Plant nucleotide-binding leucine-rich repeat receptors (NLRs) are intracellular receptors that play a key role in the plant innate immune system by sensing the presence of pathogen effectors delivered inside plant cells during pathogenesis through direct or indirect recognition. Sr35 was first identified in a landrace of the Triticum urartu relative Triticum monococcum (einkorn) and confers immunity to Pgt Ug99 in bread wheat when transferred as a transgene. Direct effector binding to the leucine-rich repeats of Sr35 results in the formation of a pentameric Sr35–AvrSr35 complex, which we term the Sr35 resistosome. Electrophysiological measurements show that the Sr35 resistosome exhibits non-selective cation channel activity.

To circumvent cell death activation for protein purification, we introduced substitutions in the N-terminal residues L15E/L19E (Sr35L15E/L19E), which are predicted to be essential for Sr35 membrane association by analogy with the ZAR1 resistosome. The final 3D reconstruction of the Sr35–AvrSr35 complex contains five receptor protomers, each bound to one effector molecule. As in the ZAR1 resistosome, five Sr35 NOD modules define the base of the circular protomer arrangement, and a helical barrel formed by the fivecoiled-coil domains is buried at the centre. Unlike ZAR1, the leucine-rich repeat (LRR) domains at the outer region do not pack against each other in the Sr35 resistosome, which might explain why this region is more flexible. The modelled ATP is nested in a groove formed by HD1 and NBD. Instead, the γ-phosphate group of the ATP forms a bidentate hydrogen bond with Sr35 NBDR157 and NBDR311. Of note, the coiled-coil domain of Sr35 contributes considerably to the interprotomer interactions: the C-terminal half of α4-helix from one protomer packs against the C-terminal sides of α2- and α4-helices of the neighbouring coiled-coil protomer. In the cryo-EM structure of the Sr35 resistosome, the EDIVD motif (Glu-Asp-Ile-Val-Asp) and the adjacent Sr35 Y74 mediate the packing of the LRR domain against the coiled-coil domain. In the cryo-EM structure, AvrSr35 binds to the very C-terminal part of the Sr35 LRR domain, supporting a direct recognition mechanism of AvrSr35 by Sr35. Nearly all residues that contribute to recognizing AvrSr35 are from the ascending lateral side of the last eight LRRs, and many of the residues interact with a single helix (α10) of AvrSr35.

>[5x]TITLEKKVRKGIESLITELKLMQAVLSKVSKVPADQLDEGVKIWAGNVKELSYQMEDIVDAFMVRVGDGGESTNPKNRVKKILKKVKKLFKNGKDLHRISAALEEVVLQAKQLAELRQRYEQEMRDTSAQTSVDPRMMALYTDVTELVGIEETRDKLINMLTEGDDWSKHPLKTISIVGFGGLGKTTLAKAAYDKIKVQFDCGAFVSVSRNPEMKKVLKDILYGLDKVKYENIHNAARDEKYLIDDIIEFLNDKRYLIVIDDIWNEKAWELIKCAFSKKSPGSRLITTTRNVSVSEACCSSEDDIYRMEPLSNDVSRTLFCKRIFSQEEGCPQELLKVSEEILKKCGGVPLAIITIASLLANKGHIKAKDEWYALLSSIGHGLTKNRSLEQMKKILLFSYYDLPSYLKPCLLYLSIFPEDREIRRARLVWRWISEGFVYSEKQDISLYELGDSYFNELVNRSMIQPIGIDDEGKVKACRVHDMVLDLICSLSSEENFVTILDDPRRKMPNSESKVRRLSIQNSKIDVDTTRMEHMRSVTVFSDNVVGKVLDISRFKVLRVLDLEGCHVSDVGYVGNLLHLRYLGLKGTHVKDLPMEVGKLQFLLTLDLRGTKIEVLPWSVVQLRRLMCLYVDYGMKLPSGIGNLTFLEVLDDLGLSDVDLDFVKELGRLTKLRVLRLDFHGFDQSMGKALEESISNMYKLDSLDVFVNRGLINCLSEHWVPPPRLCRLAFPSKRSWFKTLPSWINPSSLPLLSYLDITLFEVRSEDIQLLGTLPALVYLEIWNYSVFEEAHEVEAPVLSSGAALFPCATECRFIGIGAVPSMFPQGAAPRLKRLWFTFPAKWSSSENIGLGMRHLPSLQRVVVDVISEGASREEADEAEAALRAAAEDHPNRPILDIW;>[5x]VNFPFPKKMITESNSKDIREYLASTFPFEQQSTILDSVKSIAKVQIDDRKAFDLQLKFRQENLAELKDQIILSLGANNGNQNWQKLLDYTNKLDELSNTKISPEEFIEEIQKVLYKVKLESTSTSKLYSQFNLSIQDFALQIIHSKYKSNQISQNDLLKLITEDEMLKILAKTKVLTYKMKYFDSASKMGINKYISTEMMDLDWQFSHYKTFNDALKKNKASDSSYLGWLTHGYSIKYGLSPNNERSMFFQDGRKYAELYAFSKSPHRKIIPGEHLKDLLAKINKSKGIFLDQNALLDKRIYAFHELNTLETHFPGITSSFTDDLKSNYRKKMESVSLTCQVLQEIGNIHRFIESKVPYHSSTEYGLFSIPKIFSIPIDYKHGEKENLVSYVDFLYSTAHERILQDNSINQLCLDPLQESLNRIKSNIPVFFNL> GGAUGGCCGCCUAUGGUCGUCAAAUAAACUACGAAAGUAGGAUAAAGUGGAAUAGUAAGGUUUAGCUAUUCUGCGGUUUCAUCUUGUAAAGAUGGAGCUUGAGUAGGCAAGUGAGAUAUCAAUUUUUCUUAGUAUGUGAGGGUAACACUUUAGCAGAGGAGAAAAGUUGACUGGGUCUUUGCAGAGAUUCAGUUGAGUUCGGAAGAGCAAUAAGAAUAACUCAUAGAAUUCAAUGCGAGAGGUAGGGAACUAAUCCCUCCCUAUAAUCGCGGU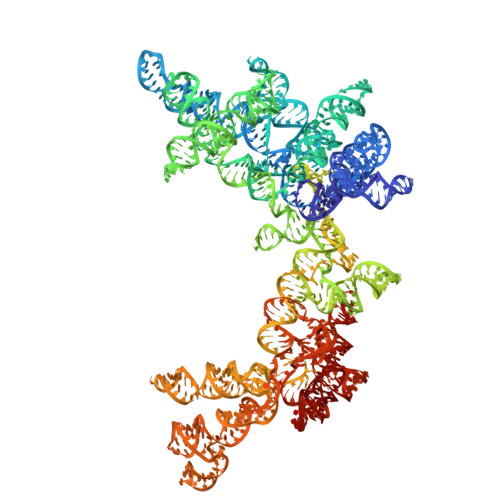AUUCAAUAUGAUAGUUUACUUAACAUCAAAUUGGGGAAACCCUUUAAGAUAAGAUAGUGUACGGGUGGUGCCGUUAUUAUCCUUUGAUAGAGUGUACCAGCACCUAUCGAUGAAGUAAACUUGGAAUAUGGUGGUAGGGAUACCACAUCGGGUAGUUAAGUAUUCUGUCGUUCAAAAGGCGGCGGAGCUUGUGAUAGACCGCUACCUGAAACCACUGCAAAACCAAACUUAUAUUUGCAUUUAGGAUUGCAAAAUCAUAAAAAUCAAAAUAAGAAAAAGUGUCUAUCAGUUUUGACCGAAAGGUGUCUACAUAGUAAUGAGUUGUUCAUUGCCACAAACACUCUCAAGGUGAAUGUGAUUCUUUCGAAAGGUUUCUAACACCGCAAGUGUGAAUCUGCUCGGCAGGGUAGAAGAAAAUAAGUAAGAAGAGAGUAGGUUAAAACUCAAAGAGUGGUUCACUUAAAUAACCGACAUUGGUUGUUACAUCUCAAAAGGAUGUGGAAACAAAGGGAAUAGAUAAUCCUUUUAAAGACAACUACAAUAUGGUGUAUUCUCAGCCU Ubiquitin-specific proteases (USPs)5 are key players in the regulation of important cellular signaling pathways through catalyzing the deconjugation reaction of ubiquitin from substrate proteins. The multifunctional protease USP15 regulates several important pathways in health and disease, including TGF-β, IGF-I, innate immune signaling, mRNA processing, and mitophagy. USP15, USP4, and USP11 share the same overall domain structure, including an N-terminal domain present in USPs (DUSP) and ubiquitin-like (UBL) domain followed by a protease domain that harbors a ∼300-amino acid insertion predicted to contain a second UBL domain. The USP15 catalytic core displays the characteristic USP protease domain fold, including a finger, palm, and thumb region.

After optimization, crystals of space group P21 diffracted to 2 Å resolution and contained one molecule in the asymmetric unit. A C-terminal tail structure unique to USP15 is rich in aromatic residues and folds back onto the catalytic core in the structure and is located on the opposite face to the distal ubiquitin S1 binding pocket. The active-site loop regions between helices α5 and α6, also referred to as the switching loop (SL; including residues Pro342–Gln353; PQFSGYQQQDCQ), and residues between β12 and β13, referred to as blocking loop 1 (BL1; residues Ser810–Arg816; SYSRYMR) that engage in USP distal ubiquitin binding are partially flexible (unrestricted by crystal contacts and not visible in the electron density; indicated as dotted lines in Fig. 1C). As a consequence, the free enzyme structure of USP15 has a largely open catalytic channel conformation for accommodating the distal ubiquitin tail that harbors the two C-terminal glycines. Interestingly, the USP15 structure shows the catalytic triad in an inactive conformation with the catalytic cysteine (Cys269) in the catalytic cleft loop between β1 and α1 (CCL; residues Ser263–Phe270; SNLGNTCF) located ∼10 Å away from the catalytic histidine (His862). In contrast to Cys269, the side chains of catalytic triad residues His862 (on β16 at the C-terminal end of BL2) and Asp879 (end of β17) are “pre-aligned” for catalysis and within hydrogen-bonding distance. Equally, residues in the blocking loop 2 between β15 and β16 (BL2; Gly856–Gly860; residues GGMGG) are partially flexible and associated with higher B-factors, suggestive of higher mobility. As a result, the ubiquitin C-terminal GG tail–binding channel is mostly open in USP15, whereas it is closed in the USP4 structure. The USP15 structure reported here displays a catalytically incompetent open conformation of the ubiquitin C-terminal tail–binding channel with active-site loops not engaged in crystal contacts, whereas a “closed” form of USP4 was previously captured with a pre-aligned catalytic triad.

> MEQPGLCGLSNLGNTCFMNSAIQCLSNTPPLTEYFLNDKYQEELNFDNPLGMRGEIAKSYAELIKQMWSGKFSYVTPRAFKTQVGRFAPQFSGYQQQDCQELLAFLLDGLHEDLNRIRKKPYIQLKDADGRPDKVVAEEAWENHLKRNDSIIVDIFHGLFKSTLVCPECAKISVTFDPFCYLTLPLASTSKVKLKDCIELFTTKEKLGAEDPWYCPNCKEHQQATKKLDLWSLPPVLVVHLKRFSYSRYMRDKLDTLVDFPINDLDMSEFLINPNAGPCRYNLIAVSNHYGGMGGGHYTAFAKNKDDGKWYYFDDSSVSTASEDQIVSKAAYVLFYQRQDTFSGTGFFPLDRETAAALEHHHHHH>[4x]GPGSMKLYDFEVGLDQPFFLIAGTCVVESEQMTIDTAGRLKEICAKLNVPFIYKSSYDKANRSSGKSFRGLGMDEGLRI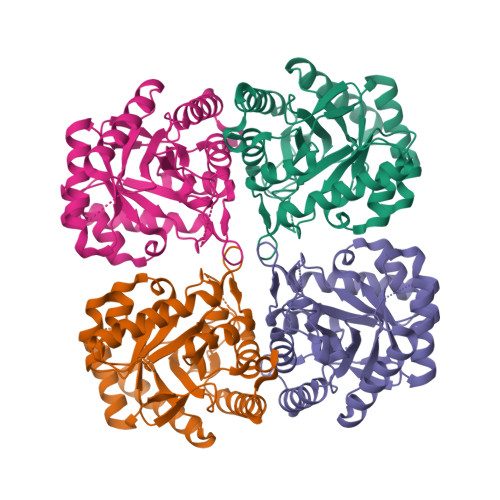LGEVKRQLGLPVLTDVHSIDEIEQVASVVDVLQTPAFLCRQTDFIHACARSGKPVNIKKGQFLAPHDMKNVIDKAREAAREAGLSEDRFMACERGVSFGYNNLVSDMRSLAIMRETSAPVVFDATHSVQLPGGQGTSSGGQREFVPVLARAAVATGVAGLFMETHPNPAEAKSDGPNAVPLNRMGALLETLVTLDQAVKRHPFLENDFN> RRG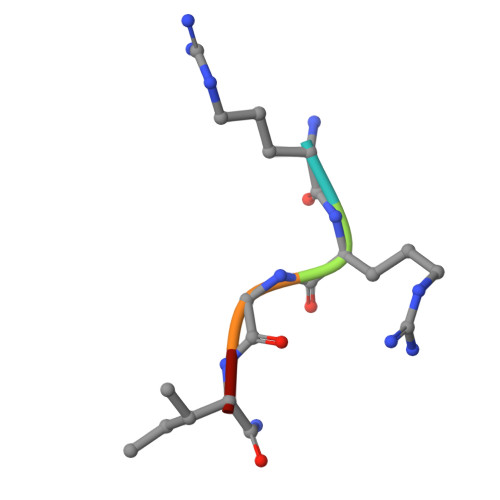IX> EDILPCVPFSVAKSVKSLYLGRMFSGTPVIRLRFKRLQPTRLVAEFDFRTFDPEGILLFAGGHQDSTWIVLALRAGRLELQLRYNGVGRVTSSGPVINHGMWQTISVEELARNLVIKVNRDAVMKIAVAGDLFQPERGLYHLNLTVGGIPFHEKDLVQPINPRLDGCMRSWNWLNGEDTTIQETVKVNTRMQCFSVTERGSFYPGSGFAFYSLDYMRTPLDVGTESTWEVEVVAHIRPAADTGVLFALWAPDLRAVPLSVALVDYHSTKKLKKQLVVLAVEHTALALMEIKVCDGQEHVVTVSLRDGEATLEVDGTRGQSEVSAAQLQERLAVLERHLRSPVLTFAGGLPDVPVTSAPVTAFYRGCMTLEV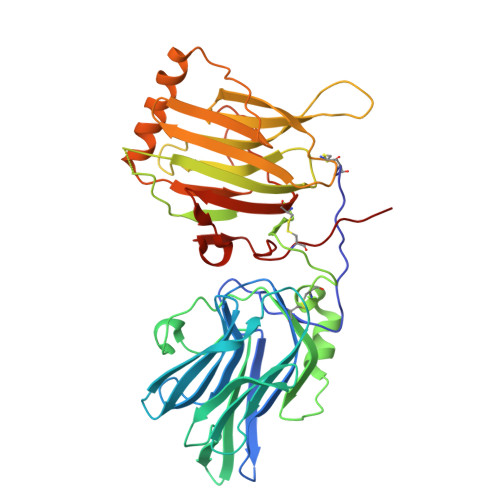NRRLLDLDEAAYKHSDITAHSCPPVEPAAA>GRKKIQITRIMDERNRQVTFTKRKFGLMKKAYELSVLCDCEIALIIFNSSNKLFQYASTDMDKVLLKYT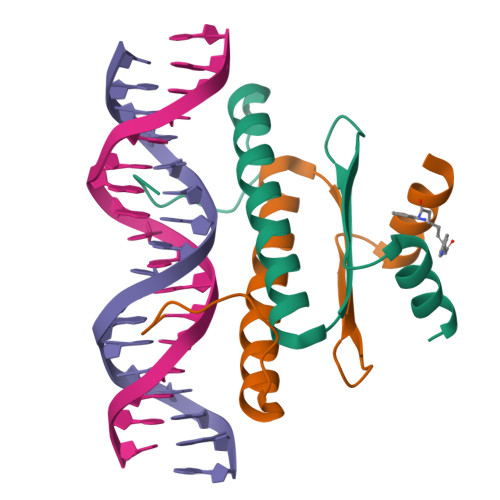AY[4x]>[12x]MLLSDRDLRAEISSGRLGIDPFDDTLVQPSSIDVRLDCLFRVFNNTRYTHIDPAKQQDELTSLVQPVDGEPFVLHPG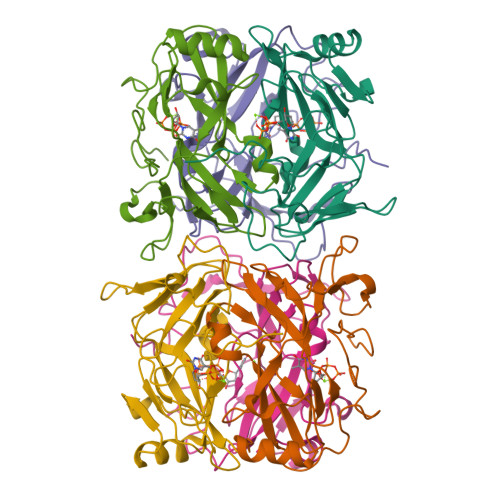EFVLGSTLELFTLPDNLAGRLEGKSSLGRLGLLTHSTVGFIDPGFSGHITLELSNVANLPITLWPGMKIGQLCMLRLTSPSEHPYGSSRAGSKYQGQRGPTPSRSYQNFIRST>[3x]GAMDPGEETINSTQNKTRTKTTRPKAVYLWTVSDVLKWYRRHCGEYTQYEQLFAQHDITGRALLRITDSSLQRMGVTDNRDREAIWREIVKQRLKTDIMEIRDMERLNIY;>GAMDPMAYINIAEWTPDQVTDWIKGLDESMKGYLYEFSKQEIGGRALLNIRPYELENLGMLRIGHQEIVLEAVENLRNFHYHLKNDNLQFMALHVATAAKNLHRELARNHAESTKIDTRILHDITRTIATLKPLVGSLERTPFRKQEMYREYCGNVLKCGLELATIAHRDRFALQPVPAIRQSAERLENLANFVIQDISDPMVLQPASLNLVTLKKRESELGFNIESSYNGIHRVTDIKYNSPAHNSGKIEDGDEIVQINYQTVVGWQHRTVLEHLREALPDVVLTVKKRPKHTKMFGQIYMQPYRLPSKKRNMAARWAAQMPSPRAAFLTLDTE[3x]

Similar to KSR, the protein Connector eNhancer of KSR (CNK) was identified by genetic means in Drosophila as a key regulatory component of the RAS–ERK pathway. In flies, CNK, like KSR, acts at a step between RAS and RAF to facilitate RAF activation, but its precise mechanism of action remains unresolved. Notably, the N-terminal part of CNK (denoted CNKNT) encompassing the SAM, CRIC and PDZ domains and a 260-residue linker preceding the PH domain can recruit the KSR–MEK complex in a manner dependent on its physical association with the SAM-domain-containing protein hyphen (HYP; also known as Aveugle). Here we show that the fly scaffold proteins CNK and HYP stabilize the KSR–MEK interaction, which in turn enhances RAF–KSR heterodimerization and RAF activation.

Given that the CNKSAM–HYPSAM domain interaction is necessary but not sufficient for KSR–MEK recruitment, we sought structural information on CNK beyond the SAM domain using CNK2–330, which minimally comprises the SAM, CRIC and PDZ domains. We determined a 2.1 Å resolution structure of the complex of CNK2–330 with HYP2–106 by single anomalous dispersion phasing using selenomethionine substituted proteins (see Extended Data Fig. 1 and Table 1 for X-ray diffraction and refinement statistics). The CNK–HYP complex adopts a rigid four-lobe torus (or ring) with extensive interactions between all four domains. As expected, the HYPSAM domain interacts with the CNKSAM domain in a prototypical head-to-tail manner with a buried contact surface of 518 Å2 described previously. A buried contact surface of 961 Å2 between HYPSAM and CNKCRIC is composed predominantly of hydrophobic residues on helix α5 of HYPSAM and on helices α2 and α3 of CNKCRIC. The PDZ domain adopts a canonical fold and, despite its C-terminal position within the SAM-CRIC-PDZ sequence, adopts a central position between the CNKSAM and CNKCRIC domains in the toroid structure, making no direct contacts with HYPSAM. Furthermore, none of the inter-domain interactions mediated by the PDZ domain are canonical in nature. A buried contact surface between CNKPDZ and CNKSAM of 667 Å2 comprises a mixture of hydrophobic and hydrophilic interactions. Importantly, this defect, as well as the reduction in pMEK levels, were fully rescued by co-introduction of the D81R mutation, which restores a favorable salt interaction but with opposite polarity. These results support the relevance of the CNKCRIC–CNKPDZ interface and provide further evidence for the validity of the toroid CNKSAM-CRIC-PDZ–HYPSAM crystal structure. Although the D195K, M197E and V198E mutations in CNK did not impair the elution profile of the CNK–HYP complex on their own, they hampered the ability of CNK–HYP to assemble with KSR–MEK. Together, these results identify a conserved surface in the vicinity of the CRIC-PDZ linker of CNK that mediates a direct interaction with KSR–MEK.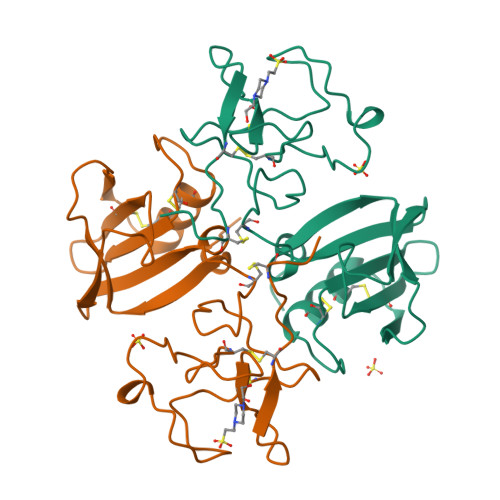>[2x]RRNTIHEFKKSAKTTLIKIDPALKIKTKKVNTADQCANRCTRNKGLPFTCKAFVFDKARKQCLWFPFNSMSSGVKKEFGHEFDLYENKDYIRNCIIGKGRSYKGTVSITKSGIKCQPWSSMIPHEHSFLPSSYRGKDLQENYCRNPRGEEGGPWCFTSNPEVRYEVCDIPQCSEVE>[2x]AECSVDIQGNDQMQFNTNAITVDKSCKQFTVNLSHPGNLPKNVMGHNWVLSTAADMQG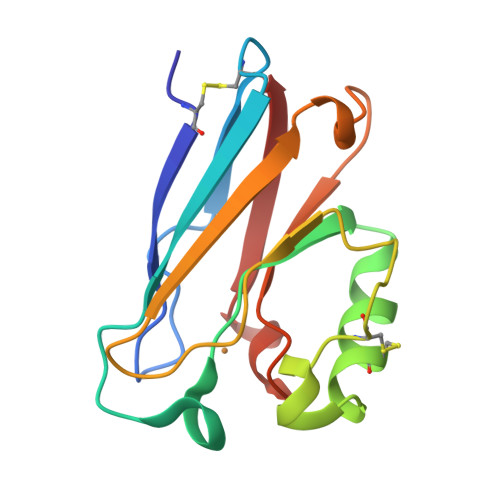VVTCGMASGLDKDYLCPDDSRVIAHTKLIGSGEKDSVTFDVSKLKGGEQYMFFCTFPGHSALMKGTLTLK> ELEFTEGIGFDKGFLSAYFVTDFDNQQAVLEDALILLHQDKISSLPDLLPLLEKVAGTGKPLLIVAEDVEGEALATLVVNAIRKTLKAVAVKGPYFGDRRKAFLEDLAVVTGGQVVNPDAGMVLREVGLEVLGSARRVVVSK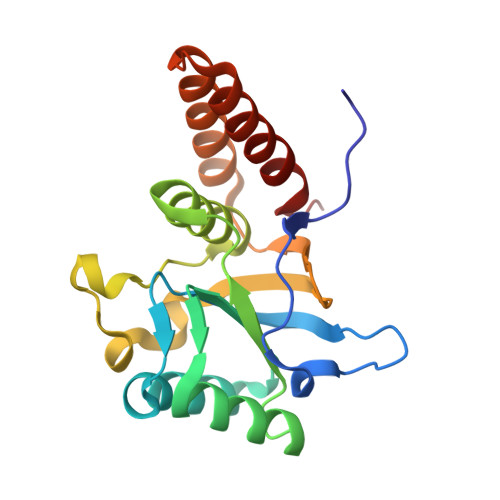DDTVIVDGGGTAEAVANRAKHLRAEIDKSDSDWDREKLGERLAKLAGGVAVI>[3x]MELESIQCDLSAFPGVKFFRIEAIFRPWRLPFVIDTLSKYGIRGLTNTPVKGVGVQGGSRERYAGTEFGPSNLVDKEKLDI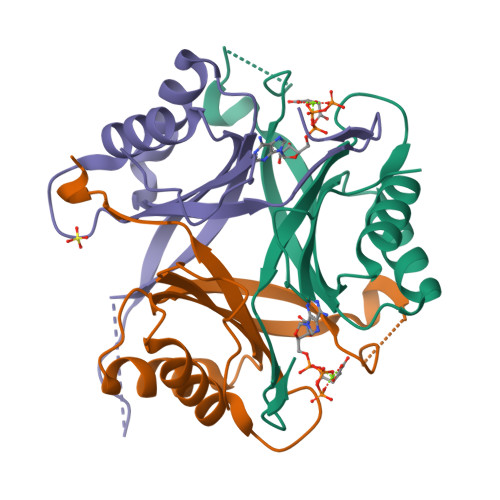VVSRAQVDAVVRLVAASAYTGEIGDGKIFVHPVAEVVRIRTAETGLEAEKMEGGMEDMMKKKKSAWSHPQFEK Endolysins are hydrolytic enzymes that specifically recognize the host cell-wall and cleave the peptidoglycan to digest the bacterial cell-wall for release of phage progeny during the lytic cycle, which is why they hold promise for the treatment of multidrug-resistant bacterial infections as an alternative to antibiotics. LysIME-EF1, an endolysin isolated from E. faecalis phage possesses a highly efficient lytic activity to multidrug resistance E. faecalis. PSI-BLAST search predicted that LysIME-EF1 consists of an N-terminal catalytic CHAP (cysteine, histidine-dependent amidohydrolases/peptidases) domain and a C-terminal CBD (cell-wall binding domain). Our finding provides structural and functional evidence that LysIME-EF1 belongs to a unique two-component multimeric endolysin encoded by a single gene.

Fortunately, we obtained diffractive crystals of selenium-labeled protein in different crystallization conditions, which were then optimized and diffracted well in the space group P1211 with cell parameters a = 47.03 Å, b = 56.92 Å, c = 91.52 Å, α = γ = 90.00°, β = 96.29°. Finally, the structure was solved successfully using the data sets belonging to the space group P1211 by selenium single-wavelength anomalous dispersion (Se-SAD) method. The crystal structure of WT LysIME-EF1 refined to 1.75 Å resolution revealed that WT LysIME-EF1 possesses a CHAP domain (residues 1–143) and a CBD (residues 168–237), which are connected by a linker (residues 144–167). The electron densities for the CHAP and the CBD domains are unambiguously defined, whereas the electron density for the linker is missing due to its high flexibility. In addition to the full-length LysIME-EF1, three additional CBD fragments were successfully built into the final model. The four CBDs together form a tetrameric ring 45 Å in length and 45 Å in width. One side of LysIME-EF1 tetrameric CBDs, which we speculate to be responsible for recognition of peptidoglycan, is arranged in a planar surface, while the other side is more convex in shape. The N-terminal CHAP domain of LysIME-EF1 folds into a typical globular domain containing two α-helices, two 310-helices and six β-strands. Analogously to LysGH15, LysIME-EF1 CHAP domain also contains a calcium-binding site and a classical amidohydrolase catalytic triad (C29, H90 and N110). Electron density of the calcium ion is clearly identified in the crystal structure, and the calcium ion is coordinated by the conserved residues D20, D22, W24, G26, D31 and one water molecule.

>[3x]MFIYYKRTKQGSTEQWFVIGGKRIYLPTMTYVNEANDLIKRYGGNTNVTTYNHDNFGLKMMEAALPQVKV;> MVKLNDVLSYVNGLVGKGVDADGWYGTQCMDLTVDVMQRFFGWRPYGNAIALVDQPLPAGFQRIRTTSSTQIKAGDVMIWGLGYYAQYGHTGIATEDGRADGTFVSVDQNWINPSLEVGSPAAAIHHNMDGVWGVIRPPYEAASTPKPPAPKPDKPNLGQFKGDDDIMFIYYKRTKQGSTEQWFVIGGKRIYLPTMTYVNEANDLIKRYGGNTNVTTYNHDNFGLKMMEAALPQVKV>GPLGSPGIPGKEILRNPMEAMDPHIFYFHFKNLRKAYGRNESWLCFTMEVVKHHSPVSWKRGVFRNQVDPETGRHAERCFLSWFADDILSPNTNYEVTWYTSWSPCPECAGEVAEFLARHSNVNLTIKTARLYYFDDTDAAEGLRSLSQEGASVEIMGYKDFKYCWENFVYNDDEPFKPWDGLDYNFLDLDSK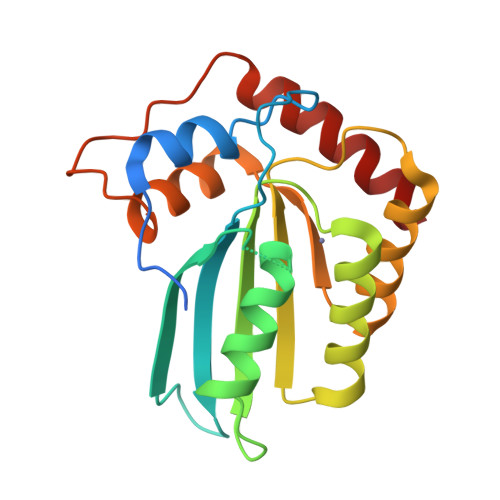LQEILE[4x]In this work, we exhaustively probe the ability of all 36 immobile HJ sequences to form DNA crystals in two different designed systems. Three separate self-assembling DNA crystal systems are described in this report: the “4 × 5” and “4 × 6” designs (collectively referred to as the 4 × N systems), and a third construct with a “scrambled” sequence variant of the 4 × 6 lattices. Self-assembly was mediated by three constituent oligonucleotides: (S1) containing four sequence repeats of either 5 or 6 bases; (S2) composed of 21 bases containing complementary regions to both (S1); and (S3) which forms the second junction crossover. The HJ serves as the fundamental component at the core of each unit, and the ultimate assembly of the full lattice is facilitated by the complementary 2-base sticky ends that tail each duplex.

Seventeen of the 36 junctions successfully crystallized, a 47% success rate. Because the 4 × 6 system yielded R3 symmetry in 5 of 17 junctions, we considered whether the downstream sequences adjacent to the junction could play a role in crystallization efficiency, junction angle, and symmetry preference, or if the HJ alone was the singular determinant. In these scenarios, R3 preferred low concentrations of divalent ions and organic solvents, and P32 required high salt with drastically different lattices. In crystals containing R3 symmetry, the average cell for each was a = b = 114.9 Å c = 49.77 Å with the c-axis confined to a tighter regime (σ = 0.75). The cavity volumes were also markedly different from the P32 cavity volumes (~614.7  nm3) compared with ~532.1 nm3 in the more densely packed R3 structure (see Supplementary Fig. 11 for calculation details). The average junction angles of 54.60° (σ = 1.44) and 58.37° (σ = 2.3) for the P32 and R3 symmetries, respectively, along with their preference for salts or organic solvents, were likely the major contributing factors that yielded the divergent lattices.

> GAGCAGACGTGA;> CGACACTCA;> TCATCG;> TCTGAGTGCGTCTGC>MARKYFVAANWKCNGTLESIKSLTNSFNNLDFDPSKLDVVVFPVSVHYDHTRKLLQSKFSTGIQNVSKFGNGSCTGEVSAEIAKDLNIEYVIIGHFERRKYFHETDEDVREKLQASLKNNLKAVVCFGESLEQREQNKTI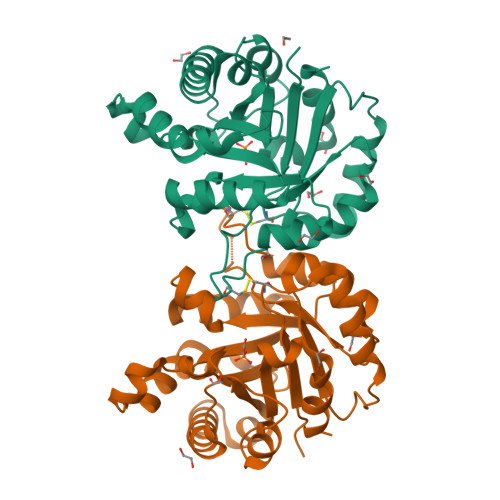EVITKQVKAFVDLIDNFDNVILVYEPLWAIGTGKTATPEQAQLVHKEIRKIVKDTCGEKQANQIRILYGGSVNTENCSSLIQQEDIDGFLVGNASLKESFVDIIKSAM[2x]> SLSCRKEQGKF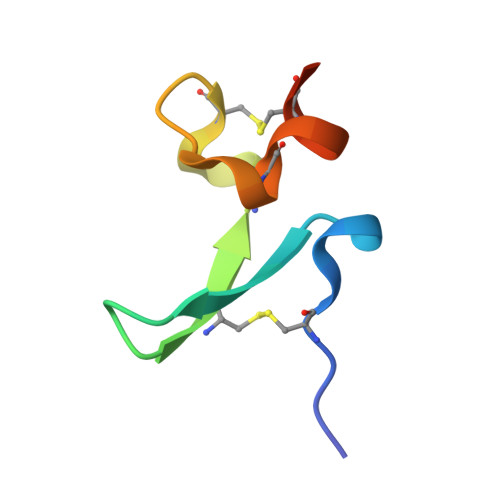YDHLLRDCISCASICGQHPKQCAYFCENKLR(METHYLPYRIDAZINE PIPERIDINE ETHYLOXYPHENYL)ETHYLACETATE | C21 H27 N3 O3 | 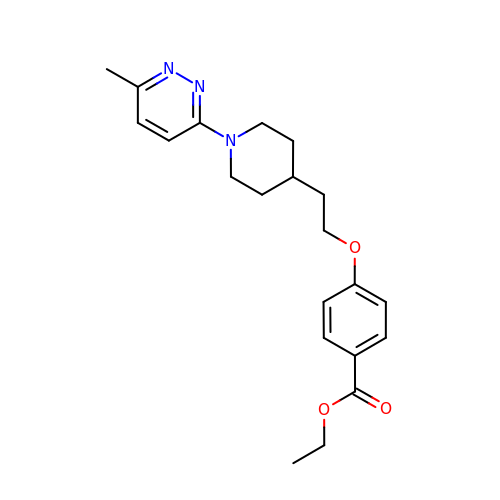KCHIOGFOPPOUJC-UHFFFAOYSA-N> PISPIETVPVKLKPGMDGPKVKQWPLTEEKIKALVEICTEMEKEGKISKIGPENPYNTPVFAIKKKDSTKWRKLVDFRELNKRTQDFWEVQLGIPHPAGLKKKKSVTVLDVGDAYFSVPLDEDFRKYTAFTIPSINNETPGIRYQYNVLPQGWKGSPAIFQSSMTKILEPFRKQNPDIVIYQYMDDLYVGSDLEIGQHRTKIEELRQHLLRWGLTTPDKKHQKEPPFLWMGYELHPDKWTVQPIVLPEKDSWTVNDICKLVGKLNWASQIYPGIKVRQLS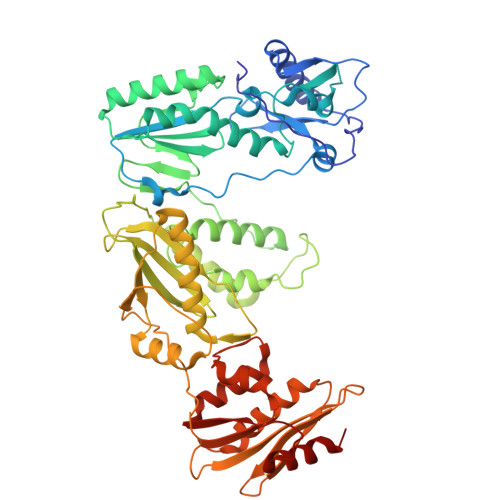KLLRGTKALTEVIPLTEEAELELAENREILKEPVHGVYYDPSKDLIAEIQKQGQGQWTYQIYQEPFKNLKTGKYARMRGAHTNDVKQLTEAVQKITTESIVIWGKTPKFKLPIQKETWETWWTEYWQATWIPEWEFVNTPPLVKLWYQLEKEPIVGAETFYVDGAANRETKLGKAGYVTNRGRQKVVTLTDTTNQKTELQAIYLALQDSGLEVNIVTDSQYALGIIQAQPDQSESELVNQIIEQLIKKEKVYLAWVPAHKGIGGNEQVDKLVSAGIRKVL>[3x]MSLKAAMPTPPVRSAAGDKEIPINGVRKAIAKHMSVSKQEIPHAWMMVEVDATGLVRYRNAVKDSFKKEEGYSLTYFAFFIKAVAQALKEFPQLNSTWAGDKIIEHANIN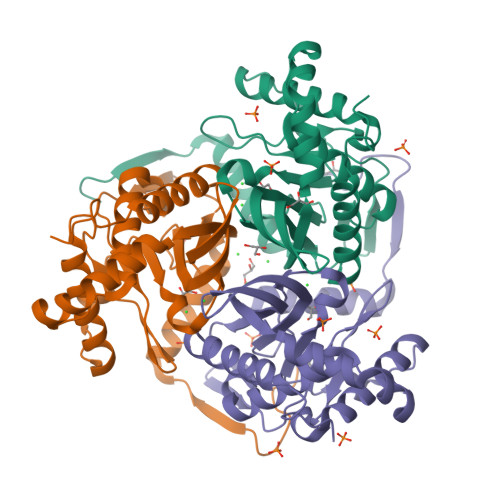ISIAIAAGDLLYVPVIKNADEKSIKGIAREISELAGKARNGKLSQADMEGGTFTVNSTGSFGSVQSMGIINHPQAAILQVESIVKRPVIIDDMIAVRDMVNLCLSIDHRILDGLLAGKFLQAIKANVEKISKENTALYEGHHHHHH>[3x]DDYSFSCYSQLEVNGSQHSLTCAFEDPDVNITNLEFEICGALVEVKCLNFRKLQEIYFIETKKFLLIGKSNICVKVGEKSLTCKKIDLTTIVKPEAPFDLSVVYREGANDFVVTFNTSHLQKKYVKVLMHDVAYRQEKDENKWTHVNLSSTKLTLLQRKLQPAAMYEIKVRSIPDHYFKGFWSEWSPSYYFRTPEI;>[3x]SVIEKLRKLEKQARKQGDEVLVMLARMVLEYLEKGWVSEEDADESADRIEEVLKK

The design of proteins that bind to a specific site on the surface of a target protein using no information other than the three-dimensional structure of the target remains a challenge. Here we describe a general solution to this problem that starts with a broad exploration of the vast space of possible binding modes to a selected region of a protein surface, and then intensifies the search in the vicinity of the most promising binding modes. We demonstrate the broad applicability of this approach through the de novo design of binding proteins to 12 diverse protein targets with different shapes and surface properties. Biophysical characterization shows that the binders, which are all smaller than 65 amino acids, are hyperstable and, following experimental optimization, bind their targets with nanomolar to picomolar affinities.

We succeeded in solving crystal structures of five of the binder–target complexes, and all five closely match the corresponding computational design models. We anticipate that the binders created here, and new ones created with the method moving forwards, will find wide utility as signalling pathway antagonists as monomeric proteins and as tuneable agonists when rigidly scaffolded in multimeric formats, and in diagnostics and therapeutics for pathogenic disease.> AVSKVYARSVYDSRGNPTVEVELTTEKGVFRSIVPSGASTGVHEALEMRDGDKSKWMGKGVLHAVKNVNDVIAPAFVKANIDVKDQKAVDDFLISLDGTANKSKLGANAILGVSLAASRAAAAEKNVPLYKHLADLSKSKTSPYVLPVPFLNVLNGGSHAGGALALQEFMIAPTGAKTFAEALRIGSEVYHNLKSLTKKRYGASAGNVGDEGGVAPNIQTAEEA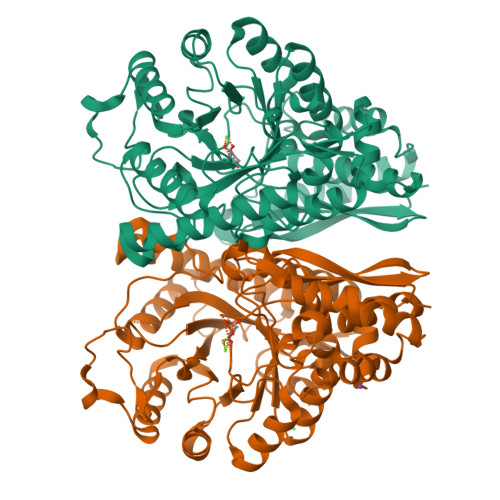LDLIVDAIKAAGHDGKVKIGLDCASSEFFKDGKYDLDFKNPNSDKSKWLTGPQLADLYHSLMKRYPIVSIEDPFAEDDWEAWSHFFKTAGIQIVADDLTVTNPKRIATAIEKKAADALLLAVNQIGTLSESIKAAQDSFAAGWGVMVSHRSGETEDTFIADLVVGLRTGQIKTGAPARSERLAKLNQLLRIEEELGDNAVFAGENFHHGDKL;> AVSKVYARSVYDSRGNPTVEVELTTEKGVFRSIVPSGASTGVHEALEMRDGDKSKWMGKGVLHAVKNVNDVIAPAFVKADIDVKDQKAVDDFLISLDGTANKSKLGANAILGVSLAASRAAAAEKDVPLYKHLADLSKSKTSPYVLPVPFLNVLNGGSHAGGALALQEFMIAPTGAKTFAEALRIGSEVYHNLKSLTKKRYGASAGNVGDEGGVAPNIQTAEEALDLIVDAIKAAGHDGKVKIGLDCASSEFFKDGKYDLDFKNPNSDKSKWLTGPQLADLYHSLMKRYPIVSIEDPFAEDDWEAWSHFFKTAGIQIVADDLTVTNPKRIATAIEKKAADALLLKVNQIGTLSESIKAAQDSFAAGWGVMVSHRSGETEDTFIADLVVGLRTGQIKTGAPARSERLAKLNQLLRIEEELGDNAVFAGENFHHGDKL> KEFEVLSFEIDEQALAFDVDNIEMVIEKSDITPVPKSRHFVEGVINLRGRIIPVVNLA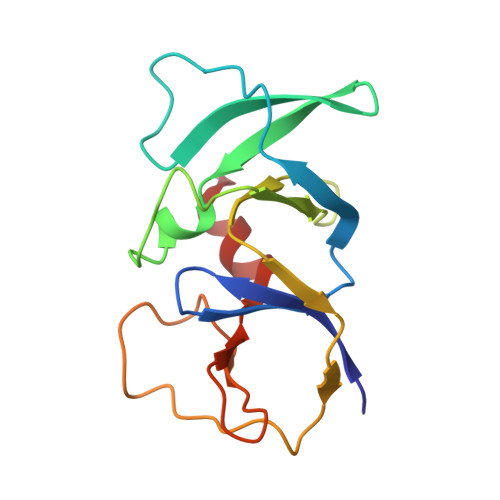KILGISFDEQKMKSIIVARTKDVEVGFLVDRVLGVLRITENQLDLTNVSDKFGKKSKGLVKTDGRLIIYLDIDKIIEEITV> AMPFEIEVLLPGEISPAETSALQKCEG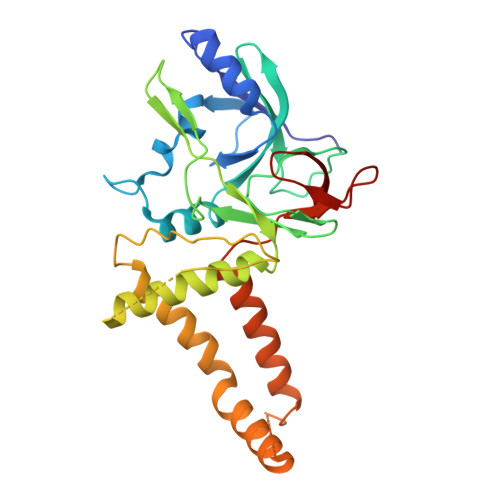KIITFSTLRHRASLVDIALSSYYINGAPPDTLSLLEAYRMRFAAVITRVIPGKLLAHAIGVGTPTPGLFIQNTSPVDLCNGDYICLLPPVFGSADEIRLDSVGLEIVFPLTIPQTLMREIIAKVVARAVERTAADVICYNGRRYELETNLQHRDGSDAAIRTLVLNLMFSINEGTTLILTLITRLLRFPIYEAISSWISTSSRLGDTLGTRAILRVCVFDGPSTVHPGDRTAVIQV> MRGSAHVVILGAGTGGMPAAYEMKEALGSGHEVTLISANDYFQFVPSNPWVGVGWKERDDIAFPIRHYVERKGIHFIAQSAEQIDAEAQNITLADGNTVHYDYLM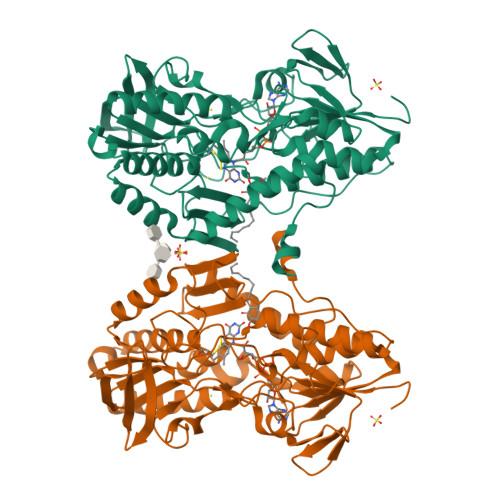IATGPKLAFENVPGSDPHEGPVQSICTVDHAERAFAEYQALLREPGPIVIGAMAGASCFGPAYEYAMIVASDLKKRGMRDKIPSFTFITSEPYIGHLGIQGVGDSKGILTKGLKEEGIEAYTNCKVTKVEDNKMYVTQVDEKGETIKEMVLPVKFGMMIPAFKGVPAVAGVEGLCNPGGFVLVDEHQRSKKYANIFAAGIAIAIPPVETTPVPTGAPKTGYMIESMVSAAVHNIKADLEGRKGEQTMGTWNAVAFADMGDRGAAFIALPQLKPRKVDVFAYGRWVHLAKVAFEKYFIRKMKMGVSEPFYEKVLFKMMGITRLKEEDTHRKAS> YV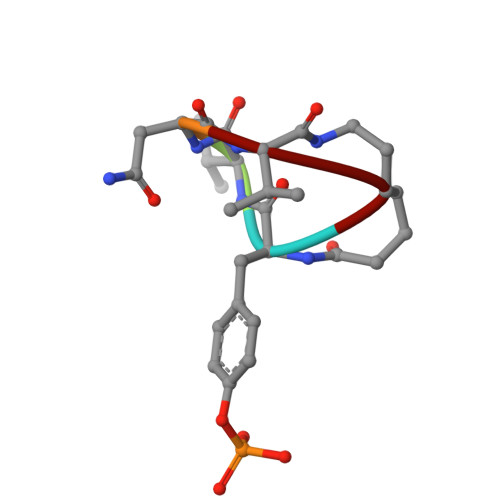NVX>[2x]MGHHHHHHGSGSNRLDGKVAIITGGTLGIGLAIATKFVEEGAKVMITGRHSDVGEKAAKSVGTPFQIQFFQHDSSDEDGWTKLFDATEKAFGPVSTLVNNAGIAVNKSVEETTTAEWRKLLAVNLDGVFFGTRLGIQRMKNKGLGASIINMSSIEGFVGDPSLGAYNASKGAVRIMSKSAALDCALKDYDVRVNTVHPGYIKTPLVDDLPG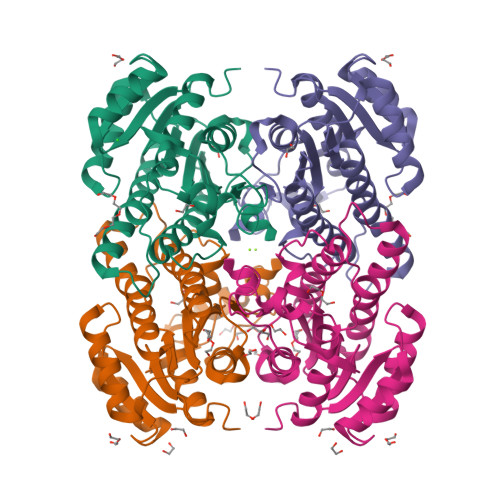AEEAMSQRTKTPMGHIGEPNDIAYICVYLASNESKFATGSEFVVDGGYTAQ> X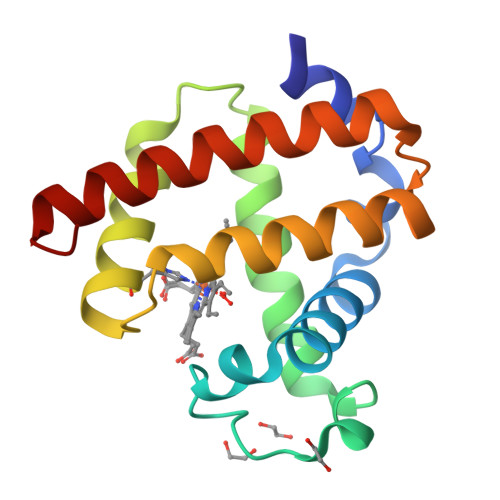ADFDAVLKCWGPVEADYTTIGGLVLTRLFKEHPETQKLFPKFAGIAQADIAGNAAVSAHGATVLKKLGELLKAKGSHAAILKPLANSHATKHKIPINNFKLISEVLVKVMQEKAGLDAGGQTALRNVMGIIIADLEANYKELGFS> ELPQMTQQLNSDDMQEQLSATVKFRQILSREHRPPIDVVIQAGVVPRLVEFMRENQPEMLQLEAAWALTNIASGTSAQTKVVVDADAVPLFIQLLYTGSVEVKEQAIWALGNVAGDSTDYRDYVLQCNAMEPILGLFNSNKPSLIRTATWTLSNLCRGKKPQPDWSVVSQALPTLAKLIYSMDTETLVDACWAISYLSDGPQEAIQAVIDVRIPKRLVELLSHESTLVQTPALRAVGNIVTGNDLQTQVVINAGVLPALRLLLSSPKENIKKEACWTISNIT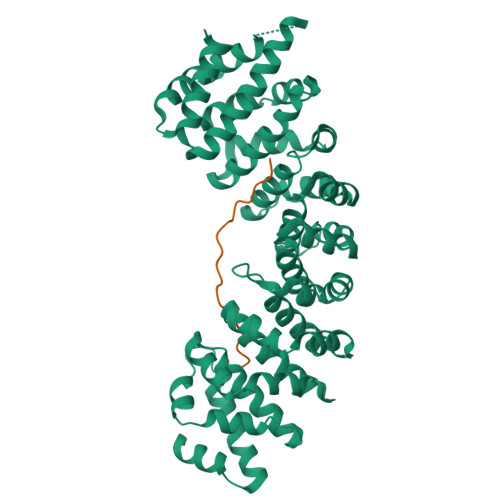AGNTEQIQAVIDANLIPPLVKLLEVAEYKTKKEACWAISNASSGGLQRPDIIRYLVSQGCIKPLCDLLEIADNRIIEVTLDALENILKMGEADKEARGLNINENADFIEKAGGMEKIFNCQQNENDKIYEKAYKIIETYFG;> SSDTRKHKFDTSTWALPNKRRRI The key enzyme is the O-acetyltransferase CsaC (MynC) encoded in region A of the CPS gene cluster. Our structural analysis of CsaC identified the capsule O-acetyltransferase of NmA as an α/β-fold enzyme with Ser-His-Asp triad. Each protomer consists of a central eight-stranded β-sheet that is sandwiched by six α-helices and capped by a lid area formed by helices α5, α6, and α7. A deep positively charged groove, which traverses the protein surface, allows substrate binding and opens into an active site that is characterized by a catalytic triad composed of S114, H228 and D198.

Consistent with the oligomeric state of CsaC in solution, the crystal packing of all CsaC structures contains a tetrameric assembly with two protein molecules in the asymmetric unit.

>[2x]MLSNLKTGNNILGLPEFELNGCRFLYKKGIEKTIITFSAFPPKDIAQKYNYIKDFLSSNYTFLAFLDTKYPEDDARGTYYITNELDNGYLQTIHCIIQLLSNTNQEDTYLLGSSKGGVGALLLGLTYNYPNIIINAPQAKLADYIKTRSKTILSYMLGTSKRFQDINYDYINDFLLSKIKTCDSSLKWNIHITCGKDDSYHLNELEILKNEFNIKAITIKTKLISGGHDNEAIAHYREYFKTIIQNILEHHHHHH>MSLNAIHRILMTTDGSITAIIEAVTQKKVEVETLEQKIIRADRELAELLEIDEGDEVNYRVVYLRANGEIYAKAISFTPLKRLENSFREDLMRADIPIGKIMRKHNIEARREIRWSRVEEADLALAKELGIADRRVISRNYNII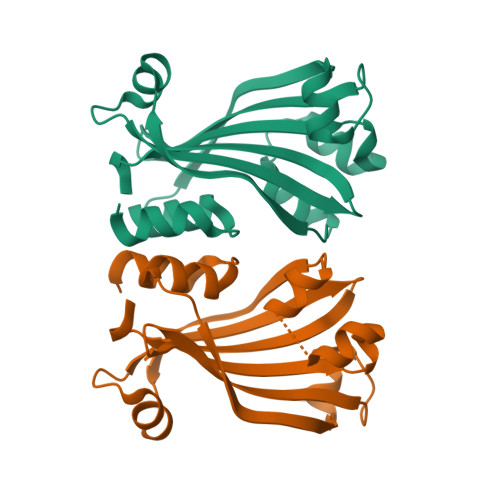HRGKVLINITEFFPMERFRIEGHHHHHH[6x]4-[5-(4-chlorophenyl)-1,3-oxazol-2-yl]benzamide | C16 H11 Cl N2 O2 | 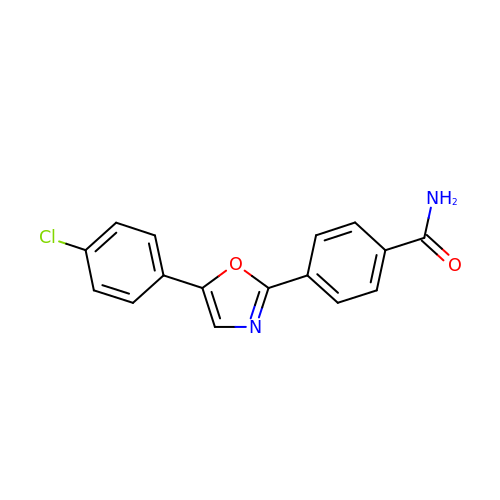DXIZWXGKFCRUNM-UHFFFAOYSA-N> HHHHHHHHAIAENAVINRLVGNWHRRAAVKREEPDVYALFDPGRPDFREDMIPFRGHPIWERLSDETRSRLLSWGWVAYNRNTVLIEQRIANPAFELVIGGAYPGLGGQQLELAVAQAMVDEQYHTLMHINGSAVTRR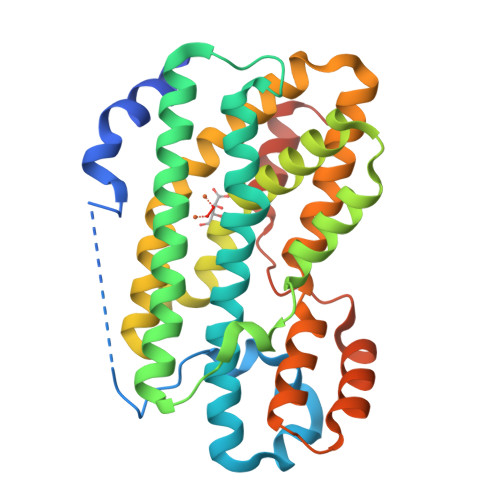MRRSDFSDRVLPDSHITTIHQEHLDRCEEPWQRSLTTLGFATVAEISINAYLDLLADDQEIQVVNSTTVKLHNRDEYCHASISGEMMKQVYEALPADRRRFLLEKVVAGLEAFVAPDFTTWESIVAFEGVPGWEKAAAEVREAQGGTHLVQDHSGIHTLLTEMDVLDQVEFGWGTTVTR>MASMGTLAFDEYGRPFLIIKDQDRKSRLMGLEALKSHIMAAKAVANTMRTSLGPNGLDKMMVDKDGDVTVTNDGATILSMMDVDHQIAKLMVELSKSQDDEIGDGTTGVVVLAGALLEEAEQLLDRGIHPIRIADGYEQAARVAIERLDKISDSVLVDIKDTEPLIQTAKTTLGSKVVNSCHRQMAEIAVNAVLTVADMERRDVDFELIKVEGKVGGRLEDTKLIKGVIVDKDFSHPQMPKKVEDAKIAILTCPFEPPKPKTKHKLDVTSVEDYKALQKYEKEKFEEMIQQIKETGANLAICQWGFDDEANHLLLQNNLPAVRWVGGPEIELIAIATGGRIVPRFSELTAEKLGFAGLVQEISFGTTKDKMLVIEQCKNSRAVTIFIRGGNKMIIEEAKRSLHDALCVIRNLIRDNRVVYGGGAAEISCALAVSQEADKCPTLEQYAMRAFADALEVIPMALSENSGMNPIQTMTEVRARQVKEMNPALGIDCLHKGTNDMKQQHVIETLIGKKQQISL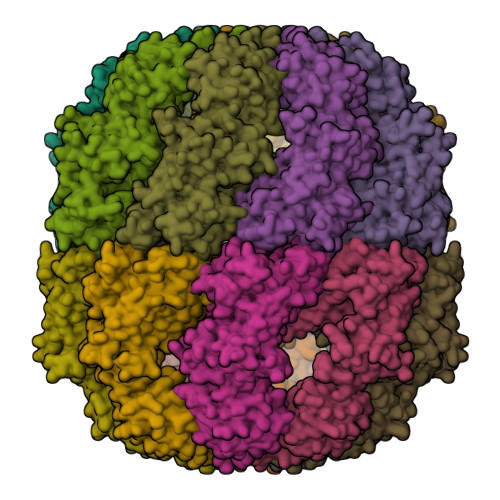ATQMVRMILKIDDIRKPGESEE[4x]N. maritimus, like most archaeal cells, is encased by a paracrystalline, proteinaceous surface layer or S-layer. The structure shows that the S-layer is pseudohexagonal and consists of the repeated interactions of the Nmar_1547 (hereafter, NmSLP) S-layer protein. At the sequence level, NmSLP is arranged into ten immunoglobulin-like (Ig-like) domains. Collectively, our structural data reveal that the S-layer of N. maritimus functions as a multichannel exchanger for ammonium ions, featuring negatively charged residues that line several pores in the S-layer.

Our goal was to solve the structure of the N. maritimus S-layer directly from whole cells. As a result, we produced a high-resolution map of the N. maritimus S-layer hexamer from intact cells. The central region of the S-layer hexamer in the map had a resolution of 3.3 Å, with the resolution decaying to around 4.5 Å towards the periphery. The subtomogram averaging map contained sufficient details to enable us to derive an atomic model of the S-layer. The first eight domains were well resolved in our 3.3–4.5-Å-resolution subtomogram averaging map. By contrast, the last two domains appeared less ordered, with the local resolution decaying towards the C terminus of NmSLP, away from the centre of the S-layer hexamer. At the N terminus, the C6 symmetry of the hexamer is broken, revealing a distinctly two-fold symmetric central pore. Each monomer of NmSLP in the S-layer adopts a rough ‘cashew’ shape, facilitating several interactions around the hexamer of NmSLP. Although the amino acid residues (37–1499) from the first eight Ig-like domains could be unambiguously built into the subtomogram averaging map, several unexplained densities were observed, emanating from surface-exposed asparagine residues. Another notable set of unexplained densities was observed near the negatively charged amino acid residue side chains of Asp73 and Glu74 at the central C2 pore, as well as between NmSLP monomers around the hexamer.

>MNNEIGRKITSLTLMTIMVAGGLTFAIPGVMPEAMAANANLFVSAENSQFDNYMSGPQVIEVVVIDSDINDTDEAKGEPDVTVNGKVLRMVQAVDGNWYGYFADRDQAQIADSTATTADSGLDFGVFCASSSGTAALGFSTTETDGIAIPITIANATATGNGTQTGSSSGGAITTTCAANTLDASTANGTINVVREAKDPVAASGSVSVGQIGLKNGTANSGPNWPFIQLYELNPTGNVVVQYNKGGGVQSTTLTFDTVDQFAELSLDRTVFPRVSQVHATITDLWLNIDPTDEDSWTFATNTKNTTSSFNVDTFYQVFDENGASGGSALTLRTTLSSLMCEDNCVLTLDVDAQSSGTPVVTIQDNGDSILTQLNASSNTNANNASAFGISTETAKLGTGSIPVTITEQGPNSGVFGTYDESDKSVLKITDNAKRGTSASLDYNETPQTILVGFSFASIDIQPVTDEWTSGQEIPVVIVDADQNKNSRADEDLDLNNPDVTLIPALRTGDPFTIDEGGTPSLIFTNGTNGDDSIFDTGAINNTSAGQVGNFTLNINVTRFSSATNITSTESIDTFSKRLISAQTANSSANFDVDFAIIDLGSATLETLKETVVDEDNTAVGFNFFNYDVRSLGADTVSIALLNTTGNILPWVNNDTRNVDKNNAILLVSNSTNSQAYVDLTNAVSDAVYGSTNTDSNVNIGFAMYFTGVGDLAAKEVIVMDFFSFGFTDDGVQSSERFANQIIRIEAEETGDNTSTFEGSLEYVMVNQINIQDAGTFSGITPIADDPSFIVIEDLTDEDAPRVNYNDLGADGVTTPVSDQEEAPSHSGVVSLNADSYKIADTVVITVEDLDLNVDSDLIDIFTVVSDNSKATDDAVGSATTQSLSFGELGRLLDVTFDDVIWSTPDGANNTATGNDSDTCSTELSNAGITDTGLGATGFTLVETGAATGVFVGDFQIPSFWCRVSDTTTTPYTYAGDEETTTGLDIEVNYVDFRDASGEIVEVGDSAGVRANTGSVSLDRTVYPVPFGTIADSSKAANAAPNGRSVFPIHATGITSTIDSTEELPTGDLTIHVRINDPDFDENPAGEDAMDQDNALKISVIRGSDSVVLGYAGASERTGKIDVGGNNGTISNIRSFGEMDEIAPDAGIFELDVNIKFTDGPASAQCNSHDTLYTALDGTTGKADTNRFDDGAASGQEYCILQGDILQVEYTDPADASGDANTVTDSATFDLRNGVLQSDKSVYIIGSDMILTLIEPDFDLDNDSAETYDLDLIEWDSDAATTTMGNKGVTGAAAAFDPEPTDFRETGDSTGIFQIVIEIPESLSNDKLERGEEIILEYTDWGPSGSDYVGDEDEDVNLTIYTSNFGATVELDQKVYSWTDKVYITIVAPDHNFDSDLVDEIGETDSDPIKVSTRGFDLDNYKLVETGTDTGIFTGEVILTGFTAHDADGDGNTGDATGTTSGSGPTDGLLATDDDDGLTVSFEFSEDETIVGSALIRWNIGEVQWLEASYPASGTGVVRVIDPDMNLDPEAVDNFEVDVWSDSDAGGIDLTVTETNEATGIFEGTVFFTTLDESSGHRLRVSEGDTVTAEYEDNTLPDPYTTADELDITATSLIGTVVPPLERAPAANLRTVDAFGNSLDSVSVDQQVQISADLANGQDREQSFAYLVQIQDANGVTVSLAWITGSLSSGQSFSPALSWIPTEAGTYTATAFVWESVDNPTALSPPVSTTVNVS[6x]> SSGAGSHCQKTSLRVNFEDIGWDSWIIAPKEYEAYECKGGCFFPLADDVTPTKHAIVQTLVHLKFPTKVSKACCVPTKLSPISVLYKDDMGVPTLKYHYEGMSVAECGCR

BMP-9 and BMP-10 are TGF-β family signaling ligands naturally secreted into blood. They act on endothelial cells and are required for proper development and maintenance of the vasculature. BMP-9 and −10 are synthesized as pro-proteins and processed by furin to release growth factors comprised of two cystine-knotted protomers that can covalently homo- or hetero-dimerize via a single cysteine in the dimer interface. Unlike other ligands of the TGF-β family, BMP-9 and −10 are secreted as a mixture of disulfide-linked dimers and monomers, in which the interchain cysteine (Cys-392) remains either paired or unpaired.

To further understand how these residues contribute to growth factor dimerization, BMP-9 G389S and BMP-9 G389S, K357R disulfide-linked dimers were crystallized at both neutral and low pH. For BMP-9 dimer mutants at neutral pH, the well solution was 1M NaCl, 22–26% glycerol, 0.1 M HEPEs pH 7.4, and the cryoprotectants ranged across 25–35% glycerol. For the crystals where the datasets were split, the integrated diffraction data was split using rebatch in the CCP4 suite to take either the first or last 32nd (or first 64th for wild type BMP-9) of diffraction images from each crystal’s 360° datasets. Where the serine is present, its sidechain hydroxyl is unstructured at neutral pH. Since wild type BMP-9 is radiation sensitive, the BMP-9 mutants were checked for radiation sensitivity. At neutral pH, the mutants lost density due to radiation damage but remained disulfide bonded. While neither mutant’s disulfide could be unambiguously modeled in a strained conformation, the radiation sensitivity demonstrates that the bonds are not ideal. While the trend is not clear between mutants at neutral pH, the damage is decreased compared to wild-type. Swapping the identified serine/glycine residues was sufficient to swap disulfide bond formation frequencies, but not equally. The interchain cystines in the variant structures reveal decreased radiation sensitivity with each additional dimerization contact.> GESQEDMFAK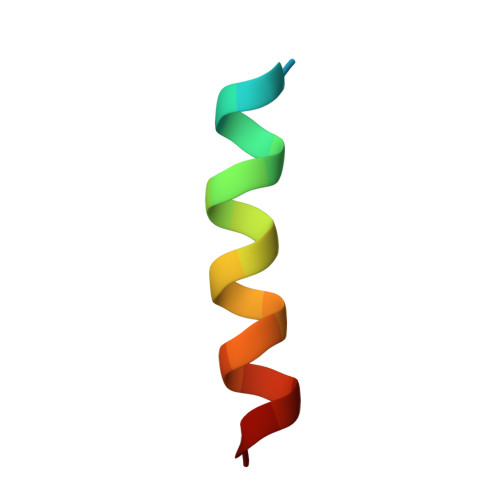LKEKLFNEINK> MNNTEENIDRIQEPTREDIDRKEAERLLDEAFNPRTKPVDRKKIINSALKILIGLYKEKKDDLTSASFISIARAYYLVSITILPKGTTIPEKKKEALRKGIEFIDRAINKFNGSILDSQRAFRIKSVLSIEFNRIDREKCDNIKLKNLL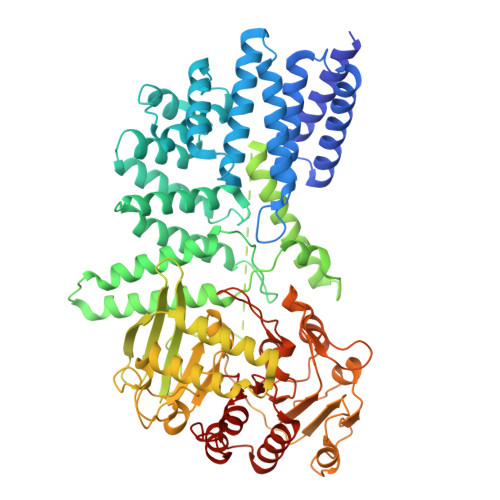NEAVDKGCTDFDTYEWDIQIAIRLCELGVDMEGHFDNLIKSNKANDLQKAKAYYFIKKDDHKAKEHMDKCTASLKYTPCSHRLWDETVGFIERLKGDSSTLWRDFAIKTYRSCRVQEKETGTLRLRWYWSRHRVLYDMAFLAVKEQADDEEPDVNVKQAKIKKLAEISDSLKSRFSLRLSDMEKMPKSDDESNHEFKKFLDKCVTAYQDGYVINRSEDKEGQGENKSTTSKQPEPRPQAKLLELTQVPEGWVVVHFYLNKLEGMGNAIVFDKCANSWQYKEFQYKELFEVFLTWQANYNLYKENAAEHLVTLCKKIGETMPFLFCDNFIPNGKDVLFVPHDFLHRLPLHGSIENKTNGKLFLENHSCCYLPAWSFASEKEASTSDEYVLLKNFDQGHFETLQNNQIWGTQSVKDGASSDDLENIRNNPRLLTILCHGEANMSNPFRSMLKLANGGITYLEILNSVKGLKGSQVILGACETDLVPPLSDVMDEHYSVATALLLIGAAGVVGTMWKVRSNKTKSLIEWKLENIEYKLNEWQKETGGAAYKDHPPTFYRSIAFRSIGFPL>[3x]TTGHSYEKYNNWETIEAWTKQVTSENPDLISRTAIGTTFLGNNIYLLKVGKPGPNKPAIFMDCGFHAREWISHAFCQWFVREAVLTYGYESHMTEFLNKLDFYVLPVLNIDGYIYTWTKNRMWRKTRSTNAGTTCIGTDPNRNFDAGWCTTGASTDPCDETYCGSAAESEKETKALADFIRNNLSSIKAYLTIHSYSQMILYPYSYDYKLPENNAELNNLAKAAVKELATLYGTKYTYGPGATTIYPAAGGSDDWAYDQGIKYSFTFELRDKGRYGFILPESQIQATCEETMLAIKYVTNYVLGHL;>RKIYAF[3x]

The carboxypeptidase TAFIa (activated thrombin activatable fibrinolysis inhibitor) is a central player in fibrinolysis. TAFIa removes carboxy-terminal lysines and arginines from partially degraded fibrin. Carboxypeptidase B (CPB) was used instead of TAFIa for practical reasons, since TAFIa was found to be highly unstable with a half-life of approximately 2h at 22 °C30. CPB, on the other hand, is stable and highly homologous to TAFIa with 48% sequence identity.

The known anabaenopeptins B, C, and F (1, 2 and 3) were isolated from a culture of the cyanobacterium Planktothrix rubescens and tested for their inhibitory activity against TAFIa in an enzymatic assay. Compounds 1–3 turned out to be potent inhibitors of TAFIa with IC50 values of 1.5, 1.9 and 1.5 nM, respectively. The comparison of 17, 3 and 14, which only differ in their R1 residues, demonstrated that Lys or Arg side chains were associated with high potency (IC50 values of 2.1 and 1.5 nM, respectively), while the Tyr residue led to a decline of activity by two orders of magnitudes (IC50 of 400 nM). In addition, we obtained crystal structures of the complexes of anabaenopeptin B (1), anabaenopeptin C (2) and anabaenopeptin F (3) with the surrogate protease carboxypeptidase B (CPB). We used CPB crystals grown in the presence of ε-caproic acid with space group P32, since these crystals had wide solvent channels, which allowed the soaking-in of large inhibitors like the anabaenopeptins. After soaking, the crystals diffracted to 2.0–2.3 Å, enabling the calculation of detailed and accurate electron density maps. The general binding modes of 1–3 were found to be very similar and in the following discussion the complex with 2 is used as an example. The linear part of the anabaenopeptins, which mimics the carboxy-terminus of the TAFIa substrate fibrin, deeply penetrated the active site channel and bound in the carboxylate- and specificity-pockets, while the circular parts of the anabaenopeptins were positioned in the entrance of the channel and completely blocked the channel like a plug, thereby preventing other molecules from entering it. All hydrogen bond donor and acceptor atoms of 2 interacted either with hydrogen bond donor/acceptors from the protein, or with bound water molecules. We found that the C-terminal arginine or lysine side chain (R1 in Fig. 3) bound in the S1’ binding pocket and interacted with the side chains of Asp255 and Ser207. The R1 residue was bound in the S1’ pocket, which is specific for basic residues like arginine and lysine in TAFIa and CPB, while the S1’ pocket of CPA is specific for large apolar residues like phenylalanine and isoleucine.> MVIVPEGTQLDEKQHIVINNGAEPQSFDPHKTEGVPESNVAYQLLEGLVTSDSEGKLQPGAAESWENTPDFKTWTFHLRKDAKWSNGDPVTAHDFVFAWRRLVDPATAAPYASYLSYLQVENAQDIIDGKKKPAELGVEAKDDYTFVVHATNPVPYAVSLTTHQSLLPLPQKVVEKLGDAWVKKENYVGNGAYKLANHIINEKIEFERNPLYWNDKETVINSATFLAIENPSTDVARYRAGDLDMTSYGLPPEQFAKLKKELLGEVYVTRTLGTYSYELNNKKAPFDNVNIRKALNLSLDRNVITDKVLGQGQTPTYVFTPTYIEEGHLIQQPAYSKEPMAQRNEEAIKLLEEAGYSKANPLKFSILYNTNENHKKVA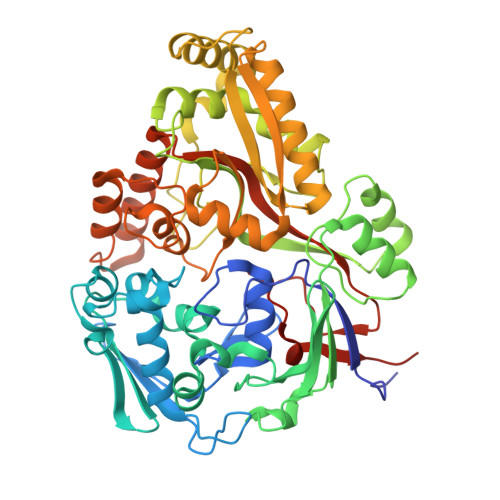IAAASMWKANTKGLIDVKLENQEWKTYIDSRRAGRYDVARAGWHADYNQATTFGNYFLSNSSNNTAKYANPEYDKAMAESYAATDAEGRAKAYAKAEEILGKDYGIVPIFNYVNPRLVKPYVKGYSGKDPQDHIYLRNLYIIKHLEHHHHHH>SNAKSAVTAQSILEKADEIRFPQDSFQVNVAIRTAAPDHAEDLYRYQVLSKGNENSIVMITEPASERGQAILMKGRDLWVFMPSVSQPIRLSLSQRLTGQVANGDIARANFTGDYHPQLLRNESIDDEDYYVLELTGIDRSVTYQKVLLWVNQSNFRPYKAEFYSVSGRLLKTSRYENFDNILGEMRPTRIIM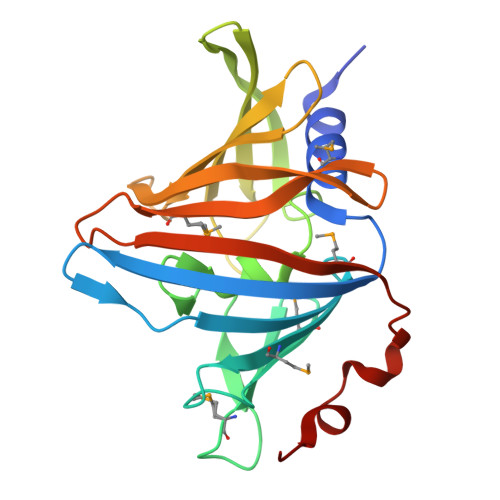EDALKSGEVSVLDYSDMKLRDLPDKIFTKDYLKRLE[2x]> GSHMPLSNFEHKVITECVTIVLGDAIQVAKCYGESVLVNAANTHLKHGGGIAGAINAASKGAVQKESDEYILAKGPLQVGDSVLLQGHSLAKNILHVVGPDARAKQDV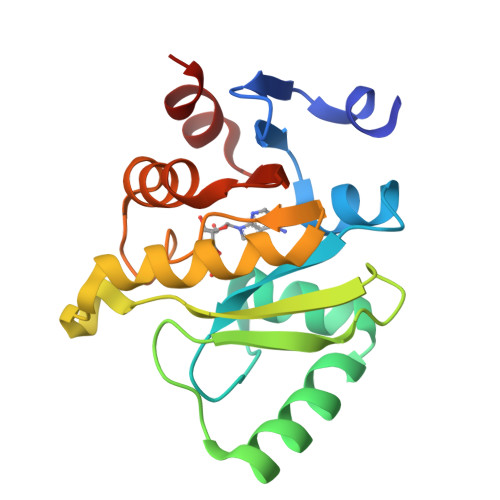SLLSKCYKAMNAYPLVVTPLVSAGIFGVKPAVSFDYLIREAKTRVLVVVNSQDVYKSLTI> MLLPDWKIRKEILIEPFSEESLQPAGYDLRVGREAFVKGKLIDVEKEGKVVIPPREYALIL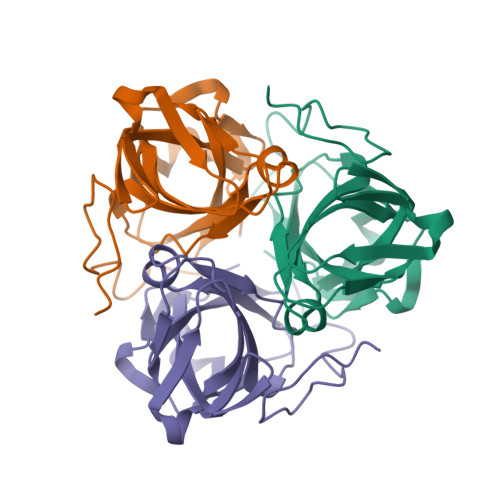TLERIKLPDDVMGDMKIRSSLAREGVIGSFAWVDPGWDGNLTLMLYNASNEPVELRYGERFVQIAFIRLEGPARNPYRGNYQGSTRLAFSKRKKL> 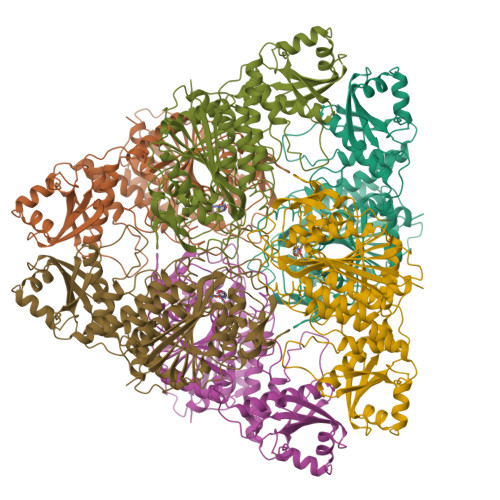XTKGLVLGIYSKEKEEDEPQFTSAGENFNKLVSGKLREILNISGPPLKAGKTRTFYGLHEDFPSVVVVGLGKKTAGIDEQENWHEGKENIRAAVAAGCRQIQDLEIPSVEVDPCGDAQAAAEGAVLGLYEYDDLKQKRKVVVSAKLHGSEDQEAWQRGVLFASGQNLARRLMETPANEMTPTKFAEIVEENLKSASIKTDVFIRPKSWIEEQEMGSFLSVAKGSEEPPVFLEIHYKGSPNASEPPLVFVGKGITFDSGGISIKAAANMDLMRADMGGAATICSAIVSAAKLDLPINIVGLAPLCENMPSGKANKPGDVVRARNGKTIQVDNTDAEGRLILADALCYAHTFNPKVIINAATLTGAMDIALGSGATGVFTNSSWLWNKLFEASIETGDRVWRMPLFEHYTRQVIDCQLADVNNIGKYRSAGACTAAAFLKEFVTHPKWAHLDIAGVMTNKDEVPYLRKGMAGRPTRTLIEFLFRFSQDSA> MDETDPILTQKNWDGTATYFQSSDEHGFSMYYKPQVGFVGDPMPFYDPVAKDFKVMYLQDYRPNPEATYHPIFGVATKDGATYESLGELISCGGRDEQDAAIGTGGTIYNPADKLYYTFYTGNKFKPSSDQNAQVVMVATSPDFKTWTKNRTFYLKGDTYGYDKNDFRDPFLFQTEDGVYHMLIATRKNGKGHIAEFTSADLKEWESAGTFMTMMWDRFYECPDVFKMGDWWYLIYSEQASFMRKVQYFKGRTLEDLKATTANDAGIWPDNREGMLDSRAFYAGKTASDGTNRYIWGWCPTRAGNDNGNVGDVEPEWAGNLVAQRLIQHEDGTLTLGVPDAIDRKYTSAQEVKVMAKDGNMIESGKTYTLGEGASVIFNRLKVHNKISFTVKTASNTDRFGISFVRGTDSASWYSIHVNADEGKANFEKDGDDAKYLFDNKFNIPADNEYRVTIYSDQSVCVTYINDQLSFTNRIYQMQKNPWSLCCYKGEITVSDVQVSTYHHHHHH

Here we introduce the first crystal structures of the B. thetaiotaomicron endo-levanase BT1760 (EC 3.2.1.65). As typical for GH32 family enzymes, the BT1760 comprises an N-terminal five-bladed β-propeller catalytic domain and a tightly packed C-terminal β-sandwich module linked to it through a short helix. The distance between the nucleophile Asp41 and the general acid/base Glu221 in the structure of BT1760 is 5.2 Å suggesting double displacement mechanism of the endo-levanase reaction with retention of the configuration of the anomeric carbon atom. For BT1760, respective amino acids are Asp41, Asp169 and Glu221.

The 508 aa-construct of endo-levanase BT1760 with C-terminal Hisx6-tag crystallized readily and yielded large (shortest dimension ~100 μm) rod-shaped crystals. While the attempts to resolve the phases using only SAD data failed, we were able to solve the structure with phenix.AutoSol in space group I222 by additionally providing an ambiguous MR solution as a partial model, or in other words, by utilizing an MR-SAD approach. A native 1.65-Å dataset was subsequently used to further refine the model. In crystallization trials, ZnCl2 emerged as an essential additive. Once the crystal structure was solved, the reason for that became evident: the protein crystallized as a 1:1 complex with Zn2+. The ion was tetragonally coordinated by His26, His384, His503 and His506, the latter two belonging to the Hisx6-tag, while His506 provided by the neighbouring symmetry-related molecule. Thus, the formed crystal actually comprises pairs of endo-levanase monomers that are linked by two closely situated Zn2+ coordination spheres, even though the asymmetric unit contains only one protein chain. In addition to the genetically removed signal peptide, the model is missing 14 residues from the N-terminus and 2 C-terminal His residues of the Hisx6-tag due to crystal disorder. Crystal structure of the wild-type BT1760 revealed a MES [2-(N-morpholino)ethanesulfonic acid] molecule in the catalytic centre with the morpholine ring of the ligand pointing towards the bottom of the active site. The morpholine ring was coordinated by two water molecules and the carbonyl oxygen of Thr104 while the ethanesulfonic acid ‘tail’ of MES was stabilized by side chains of Gln239 and Arg244.(3R,4S)-1-[(4-amino-5H-pyrrolo[3,2-d]pyrimidin-7-yl)methyl]-4-{[(4-hydroxybutyl)sulfanyl]methyl}pyrrolidin-3-ol | 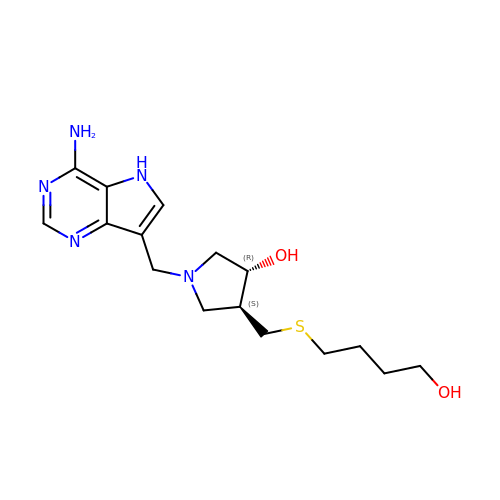C16 H25 N5 O2 S | LDGNPMXZDVLXIT-OLZOCXBDSA-N(1R,2S,3R,4R)-3-amino-4-cyclohexylcyclopentane-1,2-diol 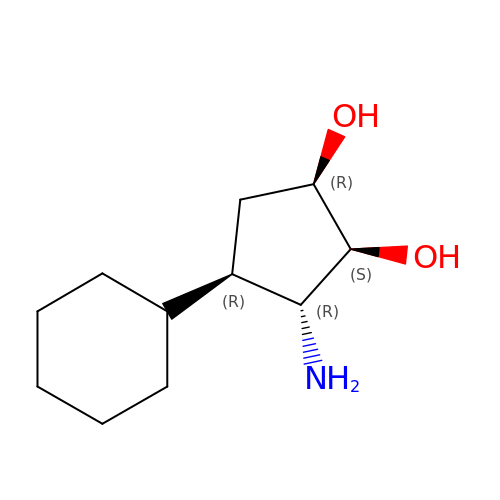| C11 H21 N O2 | CZPCDIVNIKVJDW-GWOFURMSSA-N>MTINYQFGDVDAHGAMIRAQAGLLEAEHQAIVRDVLAAGDFWGGAGSVACQEFITQLGRNFQVIYEQANAHGQKVQAAGNNMAQTDSAVGSSWATHHHHHH[2x];>[2x]SMATRFMTDPHAMRDMAGRF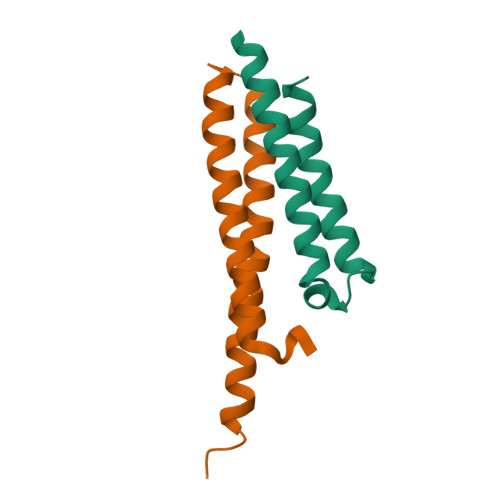EVHAQTVEDEARRMWASAQNISGAGWSGMAEATSLDTMAQMNQAFRNIVNMLHGVRDGLVRDANNYEQQEQASQQILSS>[10x]MNIIAILNHMGVYFKEEPIRELHKALEALDFQIVYPNDREDLLKLIDNNARLCGVIFDWDTYNLDLCEEISAMNEHLPVYAFANTHSTLDVSLNDLRLNVEFFEYALGAAQDIAQKIRQSTDAYIDEILPPLTKALFNYVKEGKYTFCTPGHMGGTAFQKSPVGSIFYDFFGANAMKSDISISVGELGSLLDHSGPHKEAEEYIARTFNAERSYMVTNGTSTANKIVGMYSAPAGSTVLIDRNCHKSLTHLMMMSDITPIYFRPTRNAYGILGGIPKSEFQHDTIAERVAQT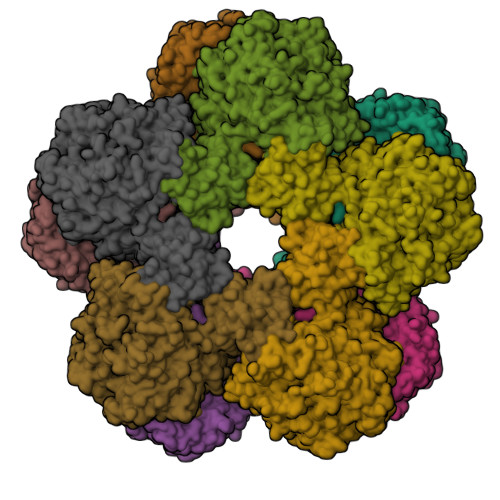PNATWPVHAVVTNSTYDGLLYNTDYIKEALDVKSIHFDSAWVPYTNFSPIYKGLCGMSGGRVEGKVIYETQSTHKLLAAFSQASMIHVKGDINEETFNEAYMMHTSTSPHYGIVASTETAAAMMKGNAGKRLINGSIERAIRFRKEIKRLNSESEGWFFDVWQPEGIDEAKCWPLDSKDNWHGFKDIDNDHMYLDPIKVTLLTPGMQKDGSMADTGIPASIVSKYLDEHGIIVEKTGPYNMLFLFSIGIDKTKALSLLRALTDFKRSYDLNLRVKNMLPSLYREDPEFYENMRIQELAQGIHALIQHHNLPDLMYRAFEVLPTMVMNPHAAFQMELRGQTEEVYLEEMIGKVNANMILPYPPGVPLVMPGEMLTEESRPVLEFLQMLCEIGAHYPGFETDIHGAYRQDGARYTVKVIK>SLEIPSKQIDYRDVFIEFLTTFKGNNNQNKYIERINELVAYRKKSLIIEFSDVLSFNENLAYEIINNTKIILPILEGALYDHILQLDPTYQ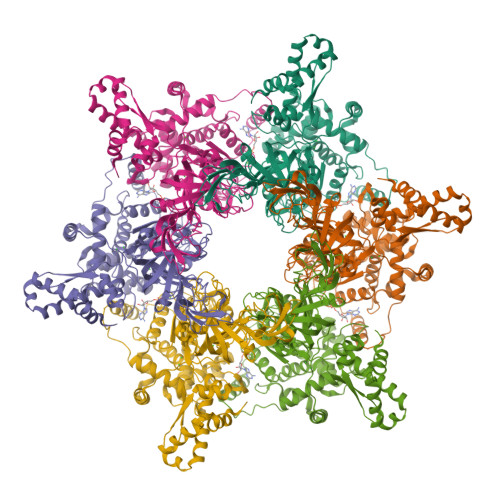RDIEKVHVRIVGIPRVIELRKIRSTDIGKLITIDGILVKVTPVKERIYKATYKHIHPDCMQEFEWPEDEEMPEVLEMPTICPKCGKPGQFRLIPEKTKLIDWQKAVIQERPEEVPSGQLPRQLEIILEDDLVDSARPGDRVKVTGILDIKQDSPVKRGSRAVFDIYMKVSSIEVSQKVLQELEISPEEEQIIKELAKRKDIVDAIVDSIAPAIYGYKEVKKGIALALFGGVSRKLPDGTRLRGDIHVLLVGDPGVAKSQILRYVANLAPRAIYTSGKSSSAAGLTAAAVRDEFTGGWVLEAGALVLADGGYALIDELDKMSDRDRSVIHEALEQQTISISKAGITATLNARTTVIAAANPKQGRFNRMKNPFEQIDLPPTLLSRFDLIFVLIDEPDDKIDSEVARHILRVRRGESEVVAPKIPHEILRKYIAYARKNIHPVISEEAMEEIEKYYVRMRKSVKKTKGEEEGIPPIPITARQLEALIRLSEAHARMRLSPIVTREDAREAIKLMEYTLKQIAMD[2x]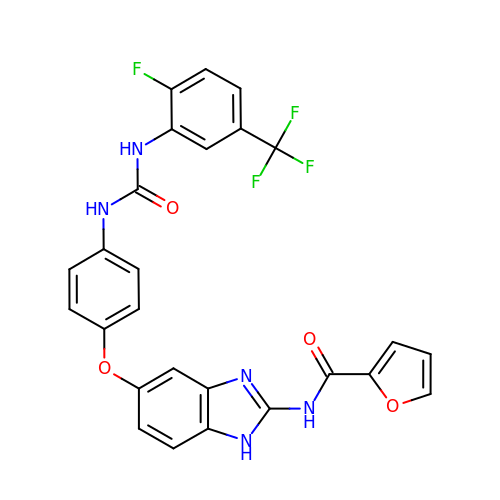~{N}-[5-[4-[[2-fluoranyl-5-(trifluoromethyl)phenyl]carbamoylamino]phenoxy]-1~{H}-benzimidazol-2-yl]furan-2-carboxamide | C26 H17 F4 N5 O4 | ODKIFGJQIHHLAP-UHFFFAOYSA-N TAGETITOXIN | C11 H17 N2 O11 P S | 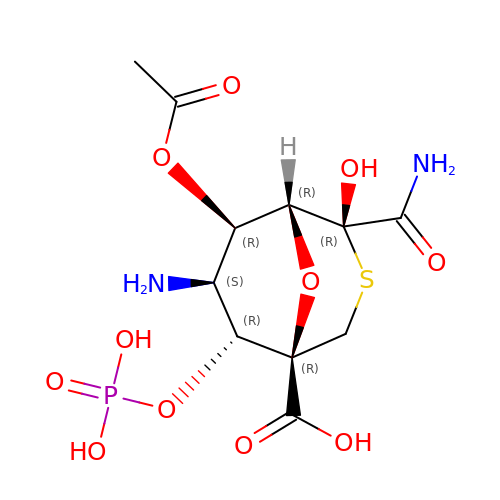UVAAUIDYGIWLMB-HGNFPZBQSA-N Here, we report on the identification, expression, biochemical and structural characterization as well as enzyme engineering of CYP109Q5 from the myxobacterium Chondromyces apiculatus DSM436. This enzyme was able to functionalize a diverse set of substrates ranging from monoterpenes over sesquiterpenes to steroids. Overall, CYP109Q5 has thus shown to accept a broad spectrum of substrates with different functionalities and size. Interestingly, CYP109Q5 showed only minimal activity with fatty acids, which distinguishes this enzyme from the CYP109 members that are actually declared as fatty acid hydroxylases, such as CYP109B1, CYP109C1, CYP109C2 or CYP109D1 (Girhard et al., 2010; Khatri et al., 2013).

In order to prepare protein for X‐ray crystallographic studies, the gene encoding CYP109Q5 was codon‐optimized for expression in E. coli and purchased from GenScript already ligated into pET‐28a(+), equipping the protein with an N‐terminal histidine tag. Crystals of CYP109Q5 diffracted to 1.55 Å and were in the P211 space group, with one monomer in the asymmetric unit. The polypeptide chain was complete except for a region G165 to A175, constituting the ‘FG loop’, which could not be modelled presumably to its mobility. The major difference between the two enzyme structures was an extended loop between N58 and P77, which, in CYP109Q5, has folded up to meet the G‐helix, possibly restricting access to the haem. The active site cavity is large and hydrophobic, with I232 and A236 at one side of the haem, and W61 and V80 brought to the other side of the substrate access channel by the movement of the N58‐P77 loop. V80 corresponds to F87 in P450 BM3, which plays a crucial role in the determination of activity and selectivity (Whitehouse et al., 2012). However, the position of W61, whose indole N atom is in contact with the haem propionate, is not a core element in the P450 superfamily and is thus special to the CYP109Q5 structure. The residue A280 is also part of the active site that is the fifth amino acid after the conserved ExxR motif the alteration of which also showed great influence on the enzyme properties. In addition, a big cavity could be seen in the surface display which presumably enables the accommodation of bulky and/or long acyclic substrates. The crystal structure of CYP109Q5 revealed flexibility within the active site pocket that permitted the accommodation of bulky substrates, and enabled a structure‐guided approach to engineering the enzyme.

> MIADIDITAPEVLRNPYALFAELRRTSAVGRLQPQGFMAVGRYQDVARVLHDAKGFSNRGWAASLPRGVKWDTSMPPSIVQVDPPRHGKLRTLVTKAFTPRTVAQLEPRIRDIAHELVDGLRGKSTFEATVEVTVPMPMIVIAEMLGVAPERRADFKRWSDDMVGSLALVRVGNAAQLERSTQEFYAYFSEVLEERRREPREDLISQLLAAEVDGEKLTAGEVLSFANTLLIAGNETTTSLIGNALVALTDHPEQLAAAQADLSLVPAVVEEVLRYESPAQCIFRQTMTDVEIGDERIPARSVVLPLLASANRDESRFPDPDRFDIHRDTKGHLAFGLDIHFCIGAPLARLEAKVMLEVLLARLGDIQRVSQEVSWSPSFFIRSPSTLPLRATVASA>MDHFNYQNDGRLFVEGLPVEQVVKKTGTPAYIYSRATIERHWQAFDSAAGKHPHLICYAVKANSNLAVLNLMARMGSGFDIVSVGELMRVIQAGGDPKKIVFSGVGKTEIEISAALQANIMCFNVESISELYRINSVAKALNVKAPISIRINPNIDAGTHPYISTGLKENKFGIEIEQALDVY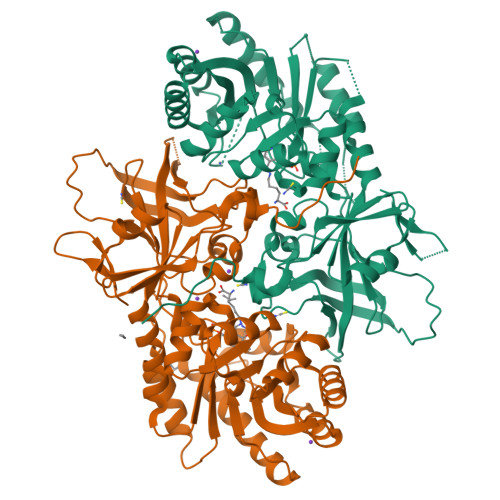KIASDLEFLEIKGVDCHIGSQLTEIAPFIEALDKLLILIDLLAEKGITISHLDLGGGLGVPYDDETPPEPAEYMTAIINRMAGRSLKLIFEPGRAIMANAGVLVTKVEFLKLNDYKNFAIVDAAMNDLIRPALYSAWQNIIPLNTDYQDGQDRPVRSYDIVGPICETGDFLGKERQLALAEGDYLVIRSTGAYGSTMSSNYNSRCRAAEILVDGEKAFIVREREELKDLWRGEHILPIHHHHHH[4x]>[4x]SHGMAVTKVTVDGIEFPPTITPPGSSKSLTLLGAGVRGVEIETIQIKMTAIGVYAEPEVIASHLQKWKGKSASELVEDDG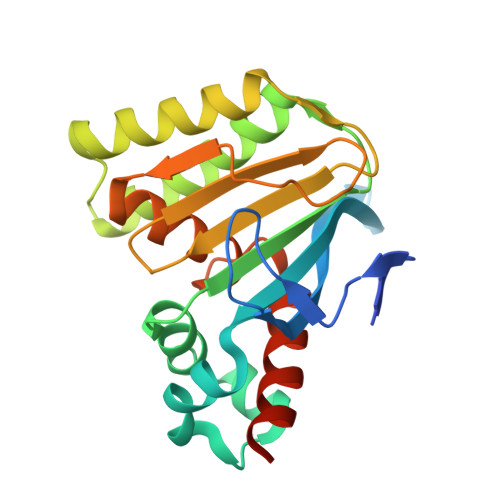FFKDLVQAPVEKLVKITIIKGFKGSQYGGALEESIRDRLAALDKYSEAEEESLEELREFFQTKSLPKGSVIFFHWPSPSTLQISVSTDGSLPEEAEATVENANVAAALLDVFLGENSVSPSTKASVAEGISALLMKNKDEKEV> GPTPMVGLDSVSG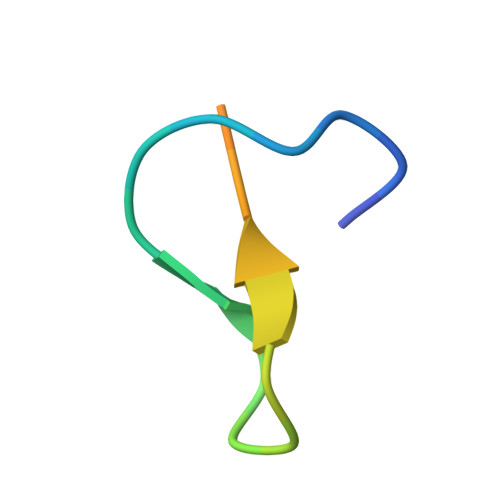QYWDQHAPLAD> W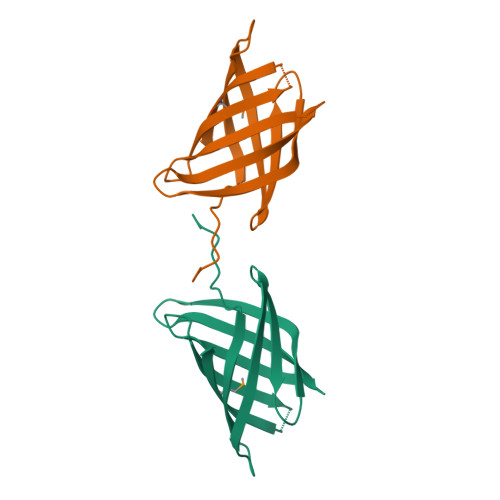QNSYLGKFLCVPNLEGRWHVDGHTRSEGGNTWEGELKIVQTWDKVRIHLKTKASHSDSVTASIIYDKGIGYQLLYNYRNQPKTGEEHLTSHVGFAEFRFDADLKSAEGHYFNGQGRATYGTMTITRIEHA> GPGSEFPDG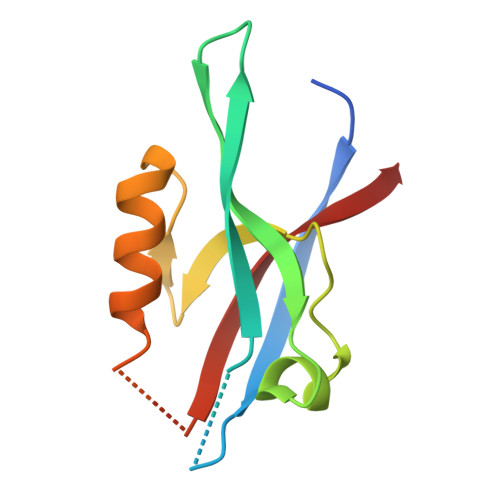TREFLTFEVPLNDSGSAGLGVSVKGNRSKENHADLGIFVKSIINGGAASKDGRLRVNDQLIAVNGESLLGKANQEAMETLRRSMSTEGNKRGMIQLIVARRIS The second primosome is the oriC-independent PriA primosome, which requires PriA to recognise the n′-pas (primosome assembly site) and initiate the primosome assembly. In general, the PriA binds to n′-pas while assisted by the auxiliary PriB, PriC, DnaT, to recruit the DnaB, DnaC and DnaG. In summary, the ssDNA binding protein DnaT, the N-terminal end of which is crucial for PriB binding, exists as a trimer in solution. Biochemical and structural information shows that the DnaT can cooperatively bind to ssDNA to form rod-like nucleoprotein filaments, which indicate that the DnaT-ssDNA complex might function as a scaffold during primosome assembly.

Although we also determined a higher resolution 1.96 Å structure, the electron density of dT10 ssDNA was very poor. Further degradations in the DnaT84–153 fragment might release the ssDNA ligand in the crystal and lead to crystal disappearance. Consequently, the incompleteness of the ligand electron density in the 1.96 Å resolution structure might be attributed to the protein degradation that caused ssDNA dissociation.

>VPMGKFAMYPDWQPDADFIRLAALWGVALREPVTTEELASFIAYWQAEGKVFHHVQWQQKLARSLQIGRASNGGLP[5x]> 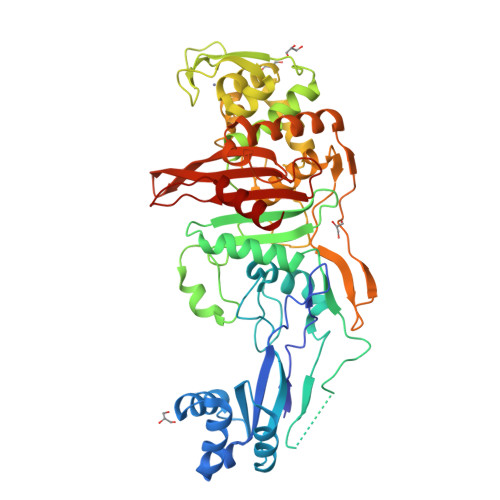GDKYKQSVESQSVEKVELNSGRGIIYDRNNKKLTDTSKSQVLIVEKEKLNNNYKILELIKKATKMNDLDIYKAVQEQLTRPIIQIQTKNIDKSMKKELEKNGIMVEEKTMRYAKDGLLSHTIGYIKEDDKSGQSGIEKSMDSVLRNSNEKYISAFKAGDAGNEKSLNILKGSVKTVDNKDKDRHLKTTIDYNIQKKLEQILNKEENPTAAIISEASTGEILAMCSRPNFDQNDISKSLKGKNGEFENRVIKATYPPGSVFKMVVLFSALENGVIDENYTYNCTGKTKVGNTNEILRCNKRDGHGFQNLRQAFSNSCNPAFLDIAMKLGKEKILKSAEKLHLFEKVDIGLDEEKIREAPKNISIRNLAIGQENIEFTPLQINQMTQIIANNGTFKPLYLYKSLVDNNMNTIKTYKSSKKEELISPYVCTQVKEYMKSVSRIGTAKDLKDIEGGCGVKTGTAQSSLNKKAIDHGWITGFYPEERPKYVITVLVEGTQKGNKSATPIFKEICESIK>[2x]MHHHHHHAMGEGVEITFNVNDYDNTLTVYTTRPDTFMGCTYLAVAAGHPLAQKAAENNPELAAFIDECRNTKVAEAEMATMEKKGVDTGFKAVHPLTG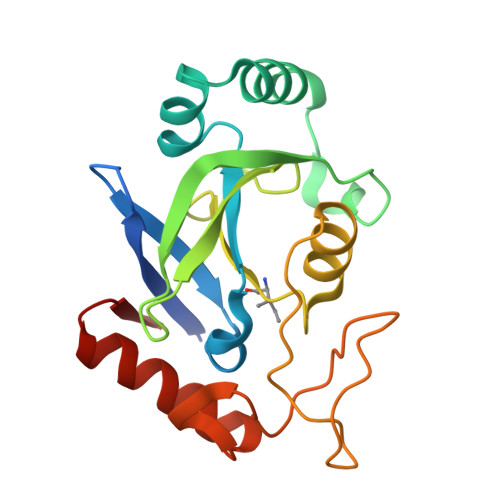EEIPVWAANFVLMEYGTGAVMAVPGHDQRDYEFASKYGLNIKPVILAADGSEPDLSQQALTEKGVLFNSGEFNGLDHEAAFNAIADKLTAMGVGERKV> MGNIMSA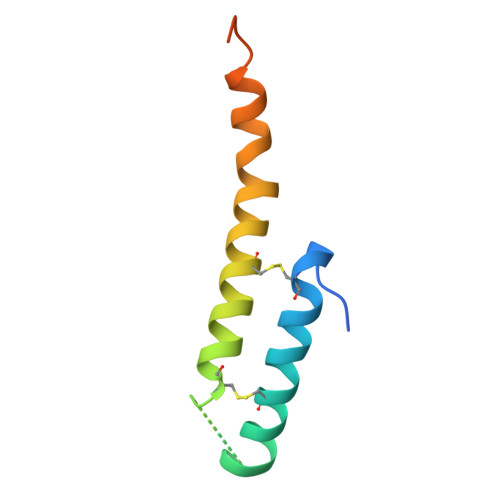SFAPECTDLKTKYDSCFNEWYSEKFLKGKSVENECSKQWYAYTTCVNAALVKQGIKPALDEAREEAPFENGGKLKEVDK>MNILLVSQCEKRALSETRRILDQFAERRGERTWQTPITQAGLDTLRRLLKKSARRNTAVACHWIRGRDHSELLWIVGDASRFNAQGAVPTNRTCRDILRKEDENDWHSAEDIRLLTVMAALFHDIGKASQAFQAKLRNRGKPMADAYRHEWVSLRLFEAFVGPGSSDEDWLRRLADKRETGDAWLSQLARDDRQSAPPGPFQKSRLPPLAQAVGWLIVSHHRLPNGDHRGSASLARLPAPIQSQWCGARDADAKEKAACWQFPHGLPFASAHWRARTALCAQSMLERPGLLARGPALLHDSYVMHVSRLILMLADHHYSSLPADSRLGDPNFPLHANTDRDSGKLKQRLDEHLLGVALHSRKLAGTLPRLERQLPRLARHKGFTRRVEQPRFRWQDKAYDCAMACREQAMEHGFFGLNLASTGCGKTLANGRILYALADPQRGARFSIALGLRSLTLQTGQAYRERLGLGDDDLAILVGGSAARELFEKQQERLERSGSESAQELLAENSHVHFAGTLEDGPLREWLGRNSAGNRLLQAPILACTIDHLMPA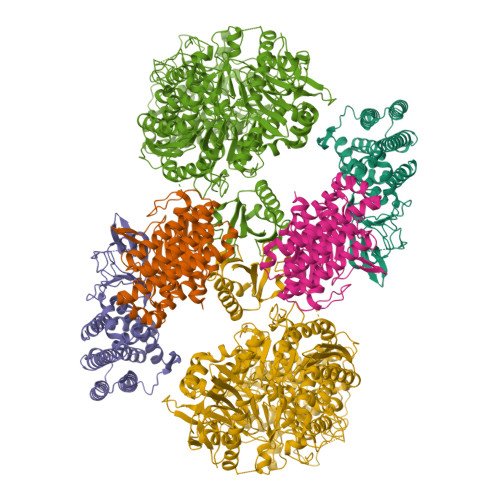SESLRGGHQIAPLLRLMTSDLVLDEVDDFDIDDLPALSRLVHWAGLFGSRVLLSSATLPPALVQGLFEAYRSGREIFQRHRGAPGRATEIRCAWFDEFSSQSSAHGAVTSFSEAHATFVAQRLAKLEQLPPRRQAQLCTVHAAGEARPALCRELAGQMNTWMADLHRCHHTEHQGRRISFGLLRLANIEPLIELAQAILAQGAPEGLHVHLCVYHSRHPLLVRSAIERQLDELLKRSDDDAAALFARPTLAKALQASTERDHLFVVLASPVAEVGRDHDYDWAIVEPSSMRSIIQLAGRIRRHRSGFSGEANLYLLSRNIRSLEGQNPAFQRPGFETPDFPLDSHDLHDLLDPALLARIDASPRIVEPFPLFPRSRLVDLEHRRLRALMLADDPPSSLLGVPLWWQTPASLSGALQTSQPFRAGAKERCYALLPDEDDEERLHFSRYEEGTWSNQDNLLRNLDLTYGPRIQTWGTVNYREELVAMAGREDLDLRQCAMRYGEVRLRENTQGWSYHPYLGFKKYN[2x];>[4x]MDDISPSELKTILHSKRANLYYLQHCRVLVNGGRVEYVTDEGRHSHYWNIPIANTTSLLLGTGTSITQAAMRELARAGVLVGFCGGGGTPLFSANEVDVEVSWLTPQSEYRPTEYLQRWVGFWFDEEKRLVAARHFQRARLERIRHSWLEDRVLRDAGFAVDATALAVAVEDSARALEQAPNHEHLLTEEARLSKRLFKLAAQATRYGEFVRAKRGSGGDPANRFLDHGNYLAYGLAATATWVLGIPHGLAVLHGKTRRGGLVFDVADLIKDSLILPQAFLSAMRGDEEQDFRQACLDNLSRAQALDFMIDTLKDVAQRSTVSA Here we show that Arabidopsis thaliana possesses a highly XMP-specific phosphatase (XMPP) which is conserved in vascular plants. We demonstrate that XMPP catalyzes the irreversible entry reaction of adenylate-derived nucleotides into purine nucleotide catabolism in vivo, whereas the guanylates enter catabolism via an unidentified GMP phosphatase and guanosine deaminase which are important to maintain purine nucleotide homeostasis. We extended the substrate survey for this enzyme to other mononucleotides and found that it is highly specific for XMP. The loop probably stabilizes the orientation of the cap domain. XMPP is a member of the Haloacid Dehalogenase (HAD) protein superfamily with unique characteristics since HAD enzymes typically have either a protruding loop or a cap structure, but not both, like XMPP.

To elucidate the molecular basis for this specificity, we determined the crystal structure of XMPP with and without XMP bound. In the complex with XMP, the 5′-monophosphate moiety of XMP provides an equatorial ligand across Asp184 in the Mg2+-coordination shell, and the ribose and xanthine moieties face toward the cap domain. Unlike the ribose moiety, xanthine embedded on the concave side of the cap domain interacts extensively with the enzyme via (i) hydrophobic interactions with Val28 and Ile32 and (ii) by base stacking with Phe55, and (iii) via direct or water-mediated indirect hydrogen bonds of O2 with Thr61, O6 indirectly with Arg51, and N3 and N7 indirectly with Tyr77 and Lys29, respectively. The interaction of Asn188 with the phosphate and of various residues with the xanthine moiety are required for full activity. Further kinetic analysis revealed that mutations of xanthine-interacting residues do not affect the kcat but the KM values for XMP. For variants altered in hydrophobic residues, the KM increases 2.2- to 26.9-fold. For those changed in hydrogen bond-forming residues, the KM increase ranges from 3.6- to 9.9-fold. The XMP specificity is thus collectively mediated by the hydrophobic residues Val28, Ile31, and Phe55 that shape the xanthine-binding pocket in the cap domain and by direct and indirect hydrogen bonds to Thr61, Lys29, and Arg51.

> MDFSPINCLIFALDDTLYPLKTGIAPAVKKNIDDFLVEKFGFSESKASSLRVELFKTYGSTLAGLRALGHDVHPDEYHSFVHGRLPYGSIEPNNKLRNLLNKIKQRKIIFTNSDKNHAVKVLKKLGLEDCFEEMICFETMNPNLFGSTTRPDEYPVVLKPSLTAMDICIRVANVDPRRTVFLDDNIHNITAGKSVGLRTILVGRAEKTKDADYAVETVTEIATAVPEIWATATATGGFDVGGERIRRSKS> GPMARTFILWLHGLGDSGPANEPIQTQFKSSELSNASWLFPSAPFNPVTCNNGAVMRSWFDVPELPLKVGSPIDESSVLEAVKNVHAIIDQEIAEGT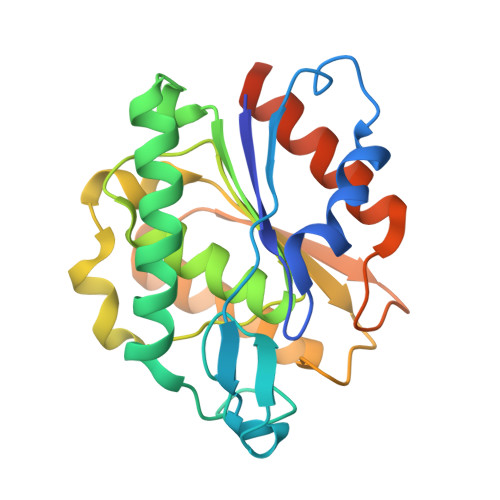NPENVFICGLSQGGALTLASVLLYPKTLGGGAVLSGWVPFTSSIISQFPEEAKKTPILWSHGTDDRMVLFEAGQAALPFLKEAGVTCEFKAYPGLGHSISNKELKYIESWIKRRLKGSSSTCLQLNCLKEMFH>MRCIGISNRDFVEGVSGGSWVDIVLEHGSCVTTMAKNKPTLDFELIKTEAKQPATLRKYCIEAKLTNTTTESRCPTQGEPSLNEEQDKRFICKHSMVDRGWGNGCGLFGKGGIVTCAKFTCKKNMEGKIVQPENLEYTIVITPHSGEEHAVGNDTGKHGKEIKITPQSSTTEAELTGYGTVTMECSPRTGLDFNEMVLLQMEDKAWLVHRQWFLDLPLPWLPGADTQGSNWIQKETLVTFKNPHAKKQDVVVLGSQEGAMHTALTGATEIQMSSG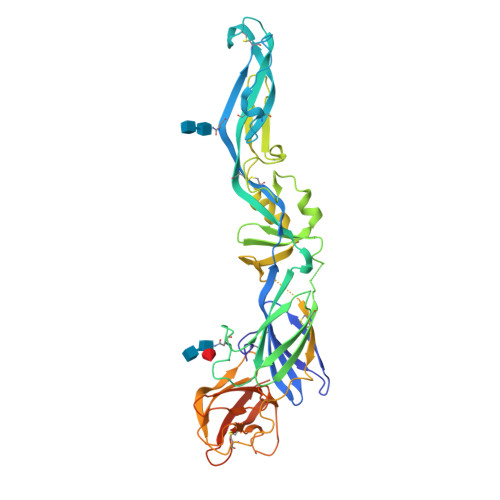NLLFTGHLKCRLRMDKLQLKGMSYSMCTGKFKIVKEIAETQHGTIVIRVQYEGDGSPCKIPFEITDLEKRHVLGRLITVNPIVTEKDSPVNIEAEPPFGDSYIIVGVEPGQLKLNWLRPLESRGPFEGKPIPNPLLGLDSTRTGHHH[2x]> GAMTFTRYSRLRVIAEIRHGDIFHSANIVSSIEFDRDDELFATAGVSRCIKVFDFSSVVNEPADMQCPIVEMSTRSKLSCLSWNKHEKN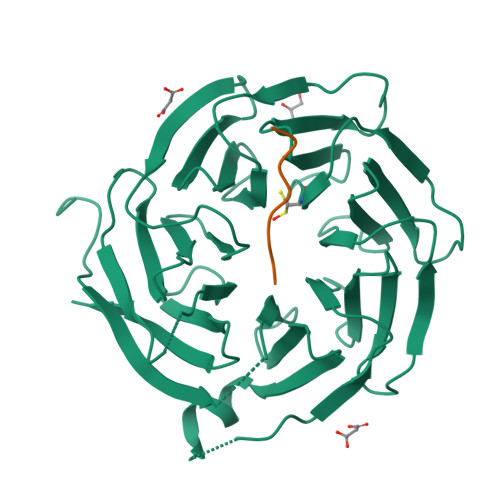HIASSDYEGIVTVWDVTTRQSLMEYEEHEKRAWSVDFSRTEPSMLVSGSDDCKVKVWCTRQEASVINIDMKANICCVKYNPGSSNYIAVGSADHHIHYYDLRNISQPLHVFSGHKKAVSYVKFLSNNELASASTDSTLRLWDVKDNLPVRTFRGHTNEKNFVGLTVNSEYLACGSETNEVYVYHKEITRPVTSHRFGSPDMDDAEEEAGSYFISAVCWKSDSPTMLTANSQGTIKVLVLAA;> XELLMVPDMY Zymogen granule membrane protein 16 (ZG16) is produced in organs that secrete large quantities of enzymes and other proteins into the digestive tract. ZG16 binds microbial pathogens, and lower ZG16 expression levels correlate with colorectal cancer, but the physiological function of the protein is poorly understood. One prominent attribute of ZG16 is its ability to bind glycans, but other aspects of the protein may also contribute to activity. An intriguing feature of ZG16 is a CXXC motif at the carboxy terminus.

Here, we describe crystal structures and biochemical studies showing that the CXXC motif is on a flexible tail, where it contributes little to structure or stability but is available to engage in redox reactions. ZG16 crystal structures also draw attention to a nonproline cis peptide bond that can isomerize within the protein and to the mobility of glycine‐rich loops in the glycan‐binding site. An understanding of the properties of the ZG16 CXXC motif and the discovery of internal conformational switches extend existing knowledge relating to the glycan‐binding activity of the protein.

>[2x]GARSSSYSGEYGSGGGKRFSHSGNQLDGPITALRVRVNTYYIVGLQVRYGKVWSDYVGGRNGDLEEIFLHPGESVIQVSGKYKWYLKKLVFVTDKGRYLSFGKDSGTSFNAVPLHPNTVLRFISGRSGSLIDAIGLHWDVYPTSCSRC> GASDPLLSVLMWGVNHSINELSHVQIPVMLMPDDFKAYSKIKVDNHLFNKENMPSHFKFKEYCPMVFRNLRERFGIDDQDFQNSLTRSAPLPNDSQARSGARFHTSYDKRYIIKTITSEDVAEMHNILKKYHQYIVECHGITLLPQFLGMYRLNVDGVEIYVIVTRNVFSHRLSVYRKYDLKGSTVAREASDKEKAKELPTLKDNDFINEGQKIYIDDNNKKVFLEKLKKDVEFLAQLKLMDYSLLVGIHDVERAEQEEVECEENDGEEEGESDGTHPVGTPPDSPGNTLNSSPPLAPGEFDPNIDVYGIKCHENSPRKEVYFMAIIDILTHYDAKKKAAHAA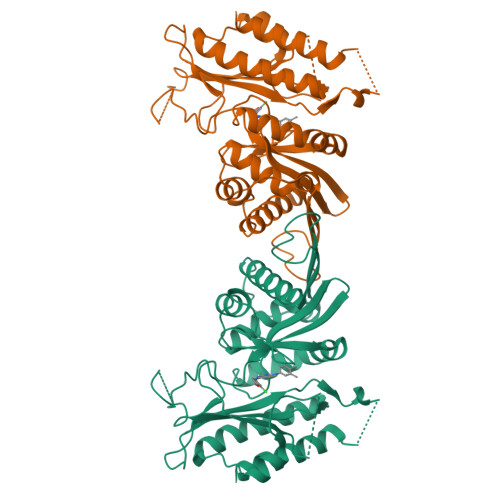KTVKHGAGAEISTVNPEQYSKRFLDFIGHILT>[4x]MKFGIEFVPNEPIQKLCYYVKLAEDNGFEYCWITDHYNNRNVYMALTAIAMNTNKIKLGPGVTNPYVRSPAITASAIATLDELSGGRAVLGIGPGDKATFDALGIEWVKPVTTLKESIEVIRKLLAGERVSYEGKVVKIAGAALAVKPIQKAVPVYMGAQGPKMLETAGMIADGVLINASNPKDFEAAIPLIKKGAEAAGRSMDEIDVAAYACMSVDKNADKAKQAAVPVVAFIAAGSPPVV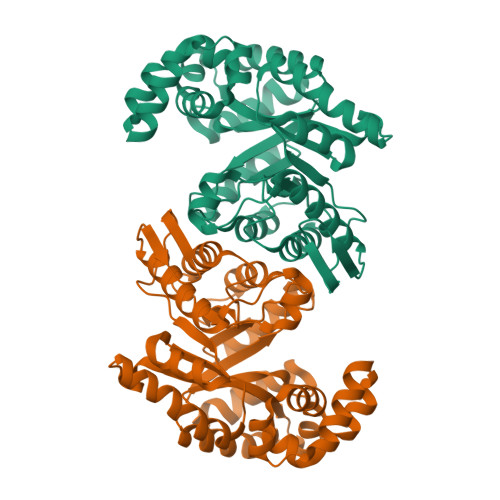LERHGIDMEKVEAIRNALKSGNFPEAFKNVDDTMLEAFSIYGTPEDVVEKCKKLAEMGVTQIVAGSPIGPNKETAIKLIGKKVIPALKEALKE> MGSSHHHHHHHHHHSSGLVPRGSHVAPPNLTREQAEQRAALLEVQSYAIELDLSAGAGGPEVETFGSTTTVRFRSATPGAESWIDLVAARVRSAVLNGVELDVSDYDESTGIRLPELAADNELVVHADCQYTNTGEGLHRFIDPVDGGVYLYSQFETADAKRMFTCFDQPDLKATYQITVTAPQDWKVISNAAGEVTDTGEGTRRHVFDTTKPMSTYLVALVAGPYAEWRDVFPGDDGQDEIPLGIYCRASLAEHLDAERLFIETKQGFGFFHKAFGVPYPFGKYDQCFVPEFNAGAMENAGCVTFLEDYVFRSRVTGYLYERRSETVLHEMAHMWFGDLVTMRWWDDLWLNESFATWASVLAQVGATQYTNAWTTFASVEKSWAYRQDQLPSTHPVAADIPDLQ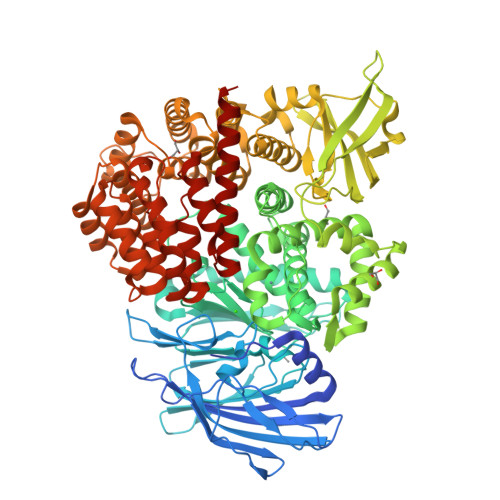AVEVNFDGITYAKGASVLKQLVAYVGLENFLAGLKVYFDRHAWGNATLDDLLVALEEASGRDLSWWSAQWLQTTGLNMLRPKLAIDDEGRFTSFSVLQSPARPGAGEHRTHRLAIGIYDDDPATGELVRTHRVELDVTGERTEVPDLVGVHRGKLVLVNDDDLTYCTMRLDPQSLATLIDRIADIQESLPRALCWSTAWEMTREAELKARDFVSLVLGSSPTTGIGAESEIGVVQRVLLQTQTALASYADPAWQPEGWRRFAGRLLELARAAEPGSDHQLAFVNSLAGSVLGEEQISAMRGWLDGTAPLEGLTVDTDLRWGLLQALVAHGAAGEAEIDAELERDQTATGRRRAERARSLIPTPEAKEKAWQRAVHDDQLPNAISDAIISGFQHPGQRELLASYVRRYFDEIDEVWHRRSSERAQPTVIGLFPSWAVDEDTVAVADRWLEGEHAPALRRLVSEGRAGIVRALAAREFDRS>[2x]MGELRVGLEESELWLRFKELTNEMIVTKNGRRMFPVLKVNVSGLDPNAMYSFLLDFVAADNHRWKYVNGEWVPGGKPEPQAPSCVYIHPDSPNFGAHWMKAPVSFSKVKLTNKLNGGGQIMLNSLHKYEPRIHIVRVGGPQRMITSHCFPETQFIAVTAYQNEEITALKIKYNPFAKAFLDAKERSHHHHHH

Brachyury is a transcription factor that plays an essential role in tumour growth of the rare bone cancer chordoma and is implicated in other solid tumours. Brachyury (encoded by the TBXT gene, also formerly known as T) is the founding member of the family and was first identified in 19275. The DNA binding domain forms an immunoglobulin-like fold and contacts DNA via an unusual insertion of an α-helix into the minor groove. All T-box proteins recognize a common consensus sequence named the T-box binding element (AGGTGTGAAA) with family member-specific variations found in the preferences for repeats, orientations (inverted or tandem), and spacing of such repeats.

We were able to crystallize the WT human brachyury DNA complex to 2.25 Å resolution using a construct spanning residues 41–224 with a 24-base pair DNA sequence. As for other T-box structures which have been obtained with near-identical DNA sequences, two copies of brachyury bind to the DNA in a 2-fold symmetrical arrangement with a small interface between subunits located towards the N-terminal end of the first β-sheet. The contact area between the two protein subunits is small (in the region of 200 Å2) and the contribution of this interface towards the possible cooperative binding on similarly spaced palindromic sites has been questioned following structures of related T-box binding proteins on the same DNA sequence which do not feature this interface. Unusually, compared to other transcription factor families which recognize sequences via major groove interactions, the final helix is inserted into the minor groove of the DNA with two conserved aromatic side chains F213 and F217 inserting deep into the groove and making contacts with the bases. As has been noted previously, only two direct hydrogen bonds are made between protein and nucleobases, R69 contacting the N7 of the guanine at position 5 of the motif, and the main chain carbonyl of F213 contacting the guanine at position 7 of the motif. The relatively high resolution of our DNA complex structures has allowed us to examine the DNA protein interface in detail including identification of water-mediated interactions. We note that a cluster of water molecules are found in this region in conserved positions when comparing our structure with the TBX3 DNA complex obtained at 1.7 Å resolution. The water network contacts the O4 of thymine at position 6, the guanine O6, and cytosine N4 at position 7. As has been found in previous T-box family DNA structures, the DNA contains some significant distortions from regular B-form geometry, most notably a widening of the minor groove to accommodate the insertion of α-4.>MVHSSAMVNSHRKPMFNIHRGFYCLTAILPQICICSQFSVPSSYHFTEDPGAFPVATNGERFPWQELRLPSVVIPLHYDLFVHPNLTSLDFVASEKIEVLVSNATQFIILHSKDLEITNATLQSEEDSRYMKPGKELKVLSYPAHEQIALLVPEKLTPHLKYYVAMDFQAKLGDGFEGFYKSTYRTLGGETRILAVTDFEPTQARMAFPCFDEPLFKANFSIKIRRESRHIALSNMPKVKTIELEGGLLEDHFETTVKMSTYLVAYIVCDFHSLSGFTSSGVKVSIYASPDKRNQTHYALQASLKLLDFYEKYFDIYYPLSKLDLIAIPDFAPGAMENWGLITYRETSLLFDPKTSSASDKLWVTRVIAHELAHQWFGNLVTMEWWNDIWLKEGFAKYMELIAVNATYPELQFDDYFLNVCFEVITKDSLNSSRPISKPAETPTQIQEMFDEVSYNKGACILNMLKDFLGEEKFQKGIIQYLKKFSYRNAKNDDLWSSLSNSCLESDFTSGGVCHSDPKMTSNMLAFLGENAEVKEMMTTWTLQKGIPLLVVKQDGCSLRLQQERFLQGVFQEDPEWRALQERYLWHIPLTYSTSSSNVIHRHILKSKTDTLDLPEKTSWVKFNVDSNGYYIVHYEGHGWDQLITQLNQNHTLLRPKDRVGLIHDVFQLVGA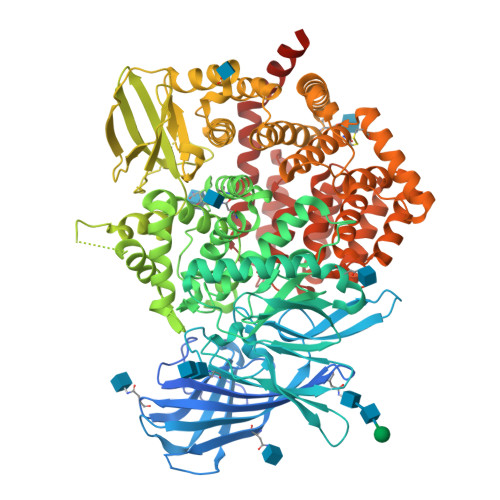GRLTLDKALDMTYYLQHETSSPALLEGLSYLESFYHMMDRRNISDISENLKRYLLQYFKPVIDRQSWSDKGSVWDRMLRSALLKLACDLNHAPCIQKAAELFSQWMESSGKLNIPTDVLKIVYSVGAQTTAGWNYLLEQYELSMSSAEQNKILYALSTSKHQEKLLKLIELGMEGKVIKTQNLAALLHAIARRPKGQQLAWDFVRENWTHLLKKFDLGSYDIRMIISGTTAHFSSKDKLQEVKLFFESLEAQGSHLDIFQTVLETITKNIKWLEKNLPTLRTWLMVNTRHHHHHH[2x]>EIIWESLSVDVGSQGNPGIVEYKGVDTKTGEVLFEREPIPIGTNNMGEFLAIVHGLRYLKERNSRKPIYSNSQTAIKWVKDKKAKSTLVRNE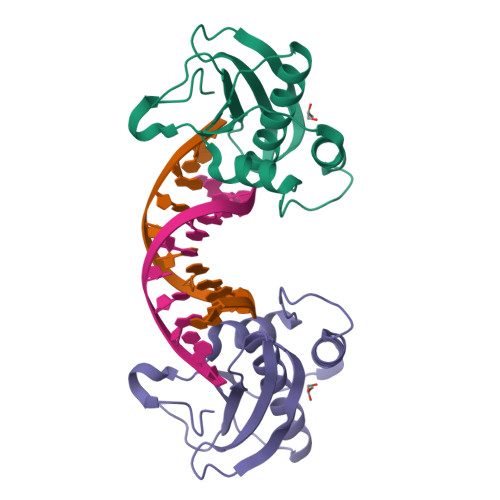ETALIWKLVDEAEEWLNTHTYETPILKWQTDKWGEIKADY[2x]>GSHMNGKLKWKFETGGSVHSSPAIGQDGTIYVGSNDHYLYAINP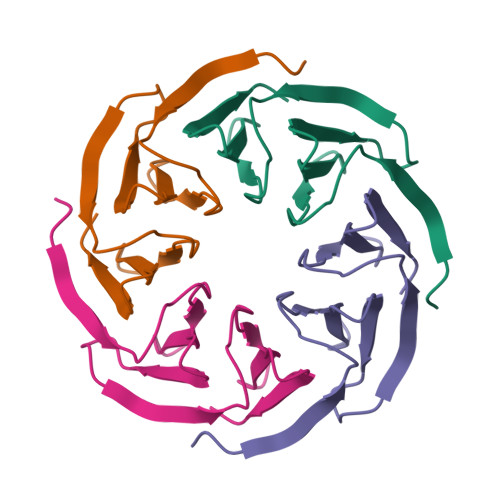NGKLKWKFETGGSVHSSPAIGQDGTIYVGSNDHYLYAINPG[8x]> GPLGSWSWESYLEEQKAITAPVSLFQDSQAVTHNKNGFKLGMKLEGIDPQHPSMYFILTVAEVCGYRLRLHFDGYSECHDFWVNANSPDIHPAGWFEKTGHKLQPPKGYKEEEFSWSQYLRSTRAQAAPKHLFVSQSHSPPPLGFQVGMKLEAVDRMNPSLVCVASVTDVVDSRFLVHFDNWDDTYDYWCDPSSPYIHPVGW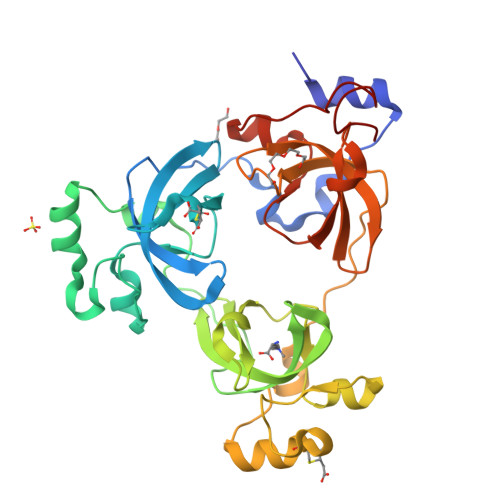CQKQGKPLTPPQDYPDPDNFCWEKYLEETGASAVPTWAFKVRPPHSFLVNMKLEAVDRRNPALIRVASVEDVEDHRIKIHFDGWSHGYDFWIDADHPDIHPAGWCSKTGHPLQPPLGGGGSAPSTGG> MGLLSILRKLKSAPDQEVR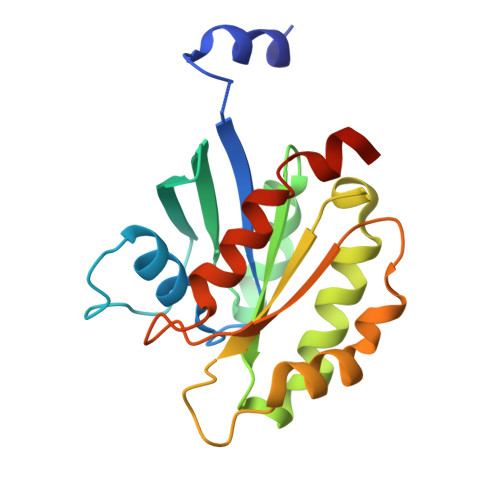ILLLGLDNAGKTTLLKQLASEDISHITPTQGFNIKSVQSQGFKLNVWDIGGQRKIRPYWRSYFENTDILIYVIDSADRKRFEETGQELTELLEEEKLSCVPVLIFANKQDLLTAAPASEIAEGLNLHTIRDRVWQIQSCSALTGEGVQDGMNWVCKNVNAKKKLEHHHHHH(2S)-2-(6-{5-[(6-aminopyridin-3-yl)sulfonyl]thiophen-2-yl}-5-chloropyridin-3-yl)-1,1,1-trifluoropropan-2-ol | C17 H13 Cl F3 N3 O3 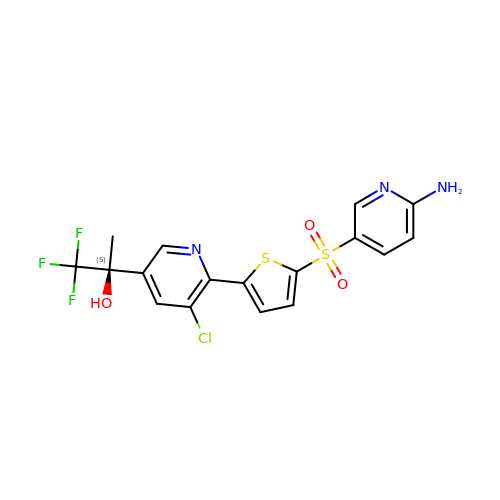S2 | KMKJDWRQGUEOJR-INIZCTEOSA-N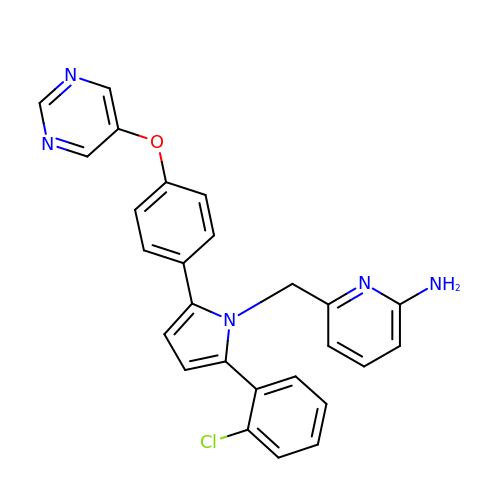6-({2-(2-chlorophenyl)-5-[4-(pyrimidin-5-yloxy)phenyl]-1H-pyrrol-1-yl}methyl)pyridin-2-amine | C26 H20 Cl N5 O | MNZJYJDKCYJKMU-UHFFFAOYSA-N> LPQSVSRAAITAAYRRPETEAVSMLLEQARLPQPVAEQAHKLAYQLADKLRNQKNASGRAGMVQGLLQEFSLSSQEGVALMCLAEALLRIPDKATRDALIRDKISNGNWQSHIGRSPSLFVNAATWGLLFTGKLVSTHNEASLSRSLNRIIGKSGEPLIRKGVDMAMRLMGEQFVTGETIAEALANARKLEEKGFRYSYDMLGEAALTAADAQAYMVSYQQAIHAIGKASNGRGIYEGPGISIKLSALHPRYSRAQYDRVMEELYPRLKSLTLLARQYDIGINIAAEESDRLEISLDLLEKLCFEPELAGWNGIGFVIQAYQKRCPLVIDYLIDLATRSRRRLMIRLVKGAYWDSE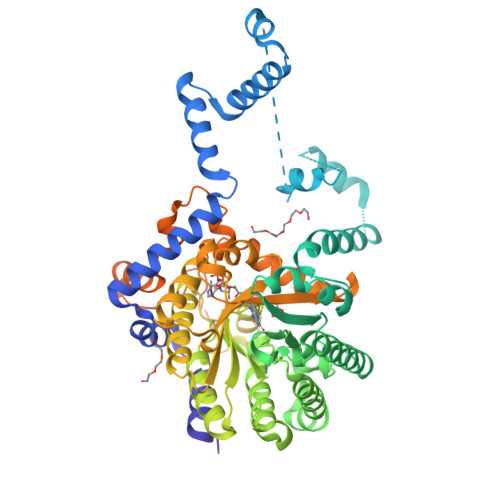IKRAQMDGLEGYPVYTRKVYTDVSYLACAKKLLAVPNLIYPQFATHNAHTLAAIYQLAGQNYYPGQYEFQCLHGMGEPLYEQVTGKVADGKLNRPCRIYAPVGTHETLLAYLVRRLLENGANTSFVNRIADTSLPLDELVADPVTAVEKLAQQEGQTGLPHPKIPLPRDLYGHGRDNSAGLDLANEHRLASLSSALLNSALQKWQALPMLEQPVAAGEMSPVINPAEPSSSVDKLAAALEHHHHHH> SLPPFKTTNLNGKIILKQGDNNCWINACCYQLQAFDFFNNEAWEKFKKGDVMDFVNLCYAATTLARGHSG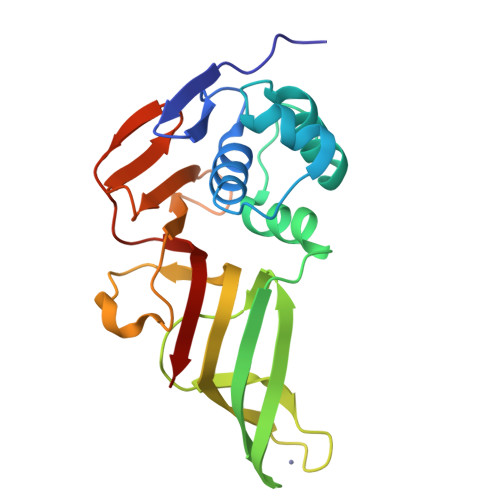DAEYLLELMLNDYSTAKIVLAAKCGCGEKEIVLERAVFKLTPLKESFNYGVCGDCMQVNTCRFLSVEGSGVFVHDILSKQTPEAMFVVKPVMHAVYTGTTQNGHYMVDDIEHGYCVDGMGIKPLKKRCYTSTLFINANVMT UvrD is classified as a SF1A helicase and plays important functions in DNA replication, recombinational repair, methyl-directed mismatch repair and nucleotide excision repair. UvrD consists of two RecA-like domains (1A and 2A) that are responsible for nucleotide binding and hydrolysis and two additional domains (1B and 2B) that are involved in dsDNA binding. Here we present crystal structures of full-length and a C-terminally truncated construct of D. radiodurans UvrD (drUvrD) in complex with 3′-tailed dsDNA. Our structures obtained in apo- and AMPPNP bound states provide us with several snapshots of this essential cellular process and reveal a large-scale spiral movement of UvrD around the duplexed DNA.

A ternary complex containing 2 molecules of intact drUvrDFL, a 21-mer DNA duplex with 7nt ssDNA extensions at each of its 3′-ends and the non-hydrolysable ATP analogue, AMPPNP, was crystallized in space group P21 with four drUvrD chains and two DNA duplexes per asymmetric unit. These crystals diffracted X-rays to 4.0 Å. Despite being present in the crystallized protein, residues 663-745 corresponding to the variable C-terminal region could not be traced in the electron density map, confirming that this region is particularly flexible. In the structures of drUvrDFL and drUvrD∆C form I, each protein monomer contains one bound AMPPNP molecule, whereas in drUvrD∆C form II each assembly is composed of a DNA duplex with an AMPPNP-bound UvrD on one end and an apo-UvrD on the other. In both drUvrDFL and drUvrD∆C form I, the two drUvrD protomers are located on the same side of the DNA duplex and induce a bend in the DNA. In the case of drUvrDFL, one of the two assemblies in the asymmetric unit forms a very bent assembly (25° bend in the DNA axis) where domains 2B of the two protomers come closer together. The second protein-DNA assembly obtained in drUvrDFL crystals is more similar to the assembly obtained in drUvrD∆C form I. In these structures, the two drUvrD protomers are still located on the same side of the DNA duplex, but the DNA duplex is less bent (16° bend in the DNA axis). In drUvrD∆C form I and drUvrDFL, the nucleotides at the junction between the dsDNA and the ssDNA are poorly defined, indicating that this region is relatively flexible. As in previous crystallographic studies of SF1 helicases, our crystal structures reveal no direct protein-protein contacts between neighboring UvrD monomers, even in the crystal structure of the intact drUvrDFL, in which the duplexed DNA is significantly bent, bringing the two UvrD monomers close to each other.

>[4x]MTSSAGPDLLQALNPTQAQAADHFTGPALVIAGAGSGKTRTLIYRIAHLIGHYGVHPGEILAVTFTNKAAAEMRERAGHLVPGAGDLWMSTFHSAGVRILRTYGEHIGLRRGFVIYDDDDQLDIIKEVMGSIPGIGAETQPRVIRGIIDRAKSNLWTPDDLDRSREPFISGLPRDAAAEAYRRYEVRKKGQNAIDFGDLITETVRLFKEVPGVLDKVQNKAKFIHVDEYQDTNRAQYELTRLLASRDRNLLVVGDPDQSIYKFRGADIQNILDFQKDYPDAKVYMLEHNYRSSARVLEAANKLIENNTERLDKTLKPVKEAGQPVTFHRATDHRAEGDYVADWLTRLHGEGRAWSEMAILYRTNAQSRVIEESLRRVQIPARIVGGVGFYDRREIRDILAYARLALNPADDVALRRIIGRPRRGIGDTALQKLMEWARTHHTSVLTACANAAEQNILDRGAHKATEFAGLMEAMSEAADNYEPAAFLRFVMETSGYLDLLRQEGQEGQVRLENLEELVSAAEEWSQDEANVGGSIADFLDDAALLSSVDDMRTKAENKGAPEDAVTLMTLHNAKGLEFPVVFIVGVEQGLLPSKGAIAEGPSGIEEERRLFYVGITRAMERLLMTAAQNRMQFGKTNAAEDSAFLEDIEGLFDTVDPYGQPIEYRAKTWKQYRPTVPAATTAVKNTSPLTAELAYRGGEQVKHPKFGEGQVLAVAGVGERQEVTVHFASAGTKKLMVKFANLTKL>[8x]MGSSHHHHHHENLYFQSNAEQVFQNFETL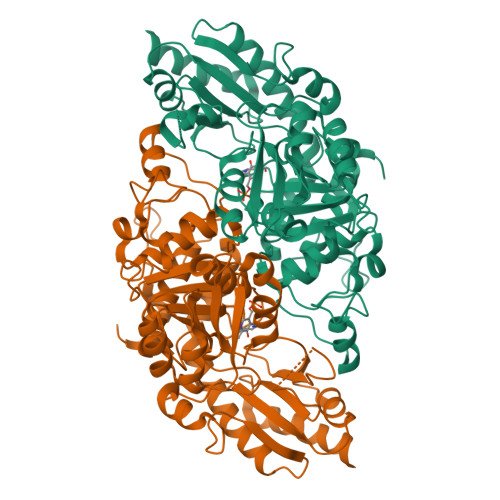QLHAGYTPDPHTRSTAVPIYATSSYTFNDSAHGARLFGLKELGNIYSRLMNPTVDVFEKRIAALEGGIAAAATSSGQAAQFLTIATLAKAGDNIVASSHLYGGTYNQLNVLLPRFGIKTKFVRSGKLEDYAAAIDDQTRAIYVESMSNPDYVVPDFEGIAKIAHEHGIPLVVDNTLGAGGYYIRPIEHGADIVVHSATKWIGGHGTTIGGVIVDSGRFNWNKHSDRFPEMVEPSPSYHGLKYWEAFGPATFITRIRVEMLRDIGACLSPFSAQQLLLGIETLGLRAERHAQNTEKLSKYFESSPNVSWVLWPGSESHPTYSQAKKYLTRGFGAMLSIGVKGDASAGSKVVDGLKLVSNLANVGDAKSLAIHPWSTTHEQLSEDERLASGVTEDMIRISVGIEHVDDIIADFEQSFQKAYGS[1-HYDROXY-2-(1,1':3',1''-TERPHENYL-3-YLOXY)ETHANE-1,1-DIYL]BIS(PHOSPHONIC 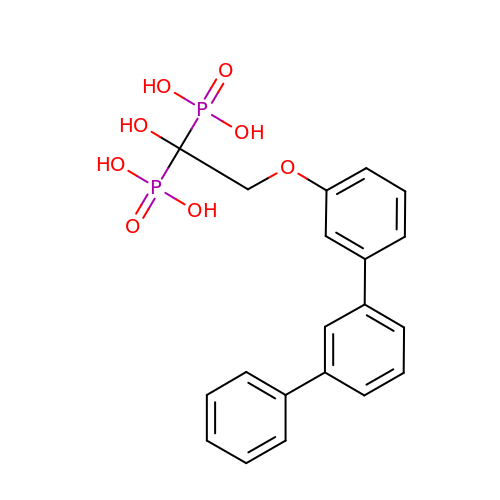ACID) | C20 H20 O8 P2 | NWIARQRYIRVYCM-UHFFFAOYSA-N> GAMGSGTARPGRSKVFNPYTEFPEFSRRLLKDLEKMFKT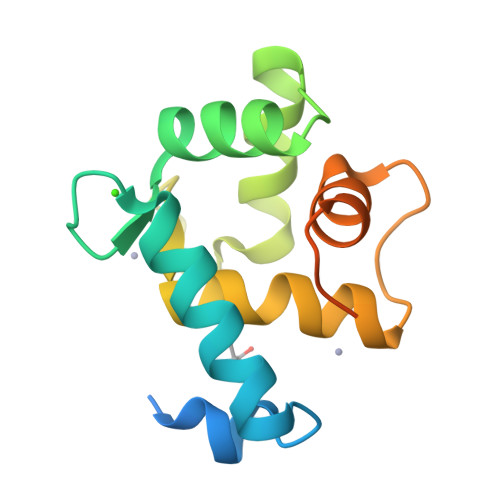YDAGRDGFIDLMELKLMMEKLGAPQTHLGLKSMIKEVDEDFDGKLSFREFLLIFHKAAAGELQEDSGLLALAKFSEIDVALEGVRGAKNFFEAKAQA KaiC is the core element of the Kai oscillator and provides a practical means for studying the essence of the clock mechanism. In the presence of KaiA and KaiB, KaiC rhythmically alters its own ATPase activity, auto-phosphorylation/auto-dephosphorylation activities, and assembly state with other Kai proteins with a period of approximately 24 h (Kai oscillator). A recent crystallographic study by our group revealed that a structural change of the C1 ring upon slow ATP hydrolysis (~11 ATP d−1) is a determinant of the period of the Kai oscillator. Using a series of KaiC mutants harboring a fluorescence probe for the C1-ring structure, we obtained evidence that the structural transition of the C1 ring is coupled with ATPase activity and the phosphorylation state and is the origin of the basic timing cue for assembly with KaiB.

Substitutions were designed to cover potential structural changes of the C1 ring, as revealed in a previous study by our group14: S157W, to monitor fraying of the α7 helix on the inner-radius side of the hexamer; S146W, to detect the cis/trans peptide isomerization near the ATPase active site; and S229W, to monitor the protomer–protomer interface on the outer-radius side of the hexamer. Therefore, the KaiC hexamer undergoes structural arrangement while maintaining the framework of the hexameric C1 ring. KaiB-induced fluorescence quenching of KaiCS157W but not KaiCWT indicates that W157, located on the inner-radius side of the C1 ring, is a sensitive probe for the conformational rearrangements that occur during assembly with KaiB. Moreover, the plot of 1/t1/2 that decreased hyperbolically with increasing the KaiB concentration is reminiscent of a conformational selection mechanism in which the conformational change in the protein occurs before ligand binding. Furthermore, exchanging external ATP with its non-hydrolyzable analog, adenylyl-imidophosphate (AMP-PNP), resulted in disappearance of the time-dependent change in FIapp after addition of KaiB. Under such solution condition, stable KaiB–KaiC complex was not detected even after long-term incubation. According to the conformational selection mechanism, the time scale of fluorescence decay at the KaiB-saturating concentration should correspond to the time scale of a conformational selection of the C1 ring before KaiB binding. Consistency between the 1/t1/2 value of ~0.5 h−1 (10.5 µM KaiB in Fig. 6c) for KaiCS157W-D/E and its ATPase activity (12 ± 1 d−1) measured in the absence of KaiB suggests that an event required in prior to KaiB binding is the slow structural change of the C1 ring from pre- into post-hydrolysis states. Taken together, the complex formation between the C1 ring and KaiB is regulated both by the phosphorylation state and by ATP hydrolysis-driven conformational change of the C1 ring to effect a rate-limiting step of the complex formation.

>[6x]MTSAEMTSPNNNSEHQAIAKMRTMIEGFDDISHGGLPIGRSTLVSGTSGTGKTLFSIQFLYNGIIEFDEPGVFVTFEETPQDIIKNARSFGWDLAKLVDEGKLFILDASPDPEGQEVVGGFDLSALIERINYAIQKYRARRVSIDSVTSVFQQYDASSVVRRELFRLVARLKQIGATTVMTTERIEEYGPIARYGVEEFVSDNVVILRNVLEGERRRRTLEILKLRGTWHMKGEYPFTITDHGINIFPLGAMRL>MGNNLMQTDLSVWGMYQHADIVVKCVMIGLILASVVTWAIFFSKSVEFFNQKRRLKREQQLLAEARSLNQANDIAADFGSKSLSLHLLNEAQNELELSEGSDDNEGIKERTSFRLERRVAAVGRQMGRGNGYLATIGAISPFVGLFGTVWGIMNSFIGIAQTQTTNLAVVAPGIAEALLATAIGLVAAIPAVVIYNVFARQIGGFKAMLGDVAAQVLLLQSRDLDLEASAAAHPVRVAQKLRAG[5x];> NVTPFIDVMLVLLIIFMVAAPL

The Ton complex is composed of three proteins ExbB, ExbD and TonB located in the inner membrane. It utilizes PMF to take up diverse compounds such as iron-loaded siderophores, haem, and vitamin B12 through outer membrane receptors. ExbB has three TM helices with a large cytoplasmic domain, and both ExbD and TonB are predicted to have single TM helices and a compact periplasmic domain. ExbB and ExbD together form a proton channel, and isolated ExbBD complexes show ion conductivity and cation selectivity in vitro.

We also reconstructed a 3D structure of the pentameric complex at pH 5.4 in the same way. The 3D map resolved a pentameric structure with clear three long α-helices per subunit in the cytoplasmic domain but poorer masses in the TM region except for a rod-like density inside the channel. Five-fold symmetrization, however, gave a better map. Although the quality of this pentamer map, particularly the continuity of α-helices at the periplasm, is still not quite as good as those of the hexameric complex, a single rod-like density appears again inside the channel in the TM region. The rod probably corresponds to the TM helix of ExbD. There is insufficient space to accommodate more helices in the channel. The arrangement of the ExbB models in the ExbB pentamer with one ExbDTM (ExbB5ExbD1TM) shows little change from the crystal structure. The crystal structure at pH 4.5 and our cryo-EM reconstruction of the pentameric complex show a central single TM helix of ExbD, which makes a ~2 Å pore at the shortest diameter. The ExbBD complex has been shown to be a cation-selective channel, but this pore size is too small for permeation of cations unless there are large fluctuations of the central helix. Thus, the structure of this pentameric complex suggests a low efficiency, blocked or semi-blocked, energy transducing state.> GGGAEALELLEHCGV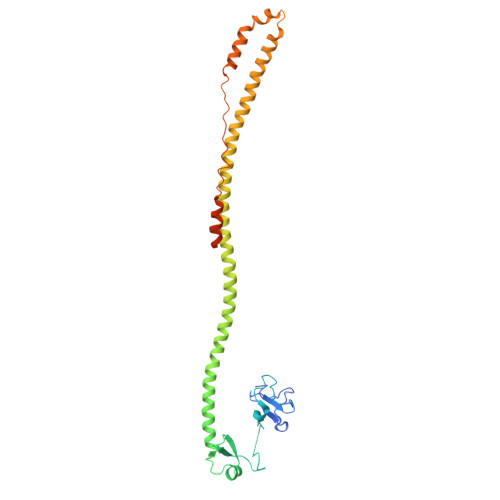CRERLRPEREPRLLPCLHSACSACLGPAAPAAANSSGDGGAAGDGTVVDCPVCKQQCFSKDIVENYFMRDSGSKAGERTVYCNVHKHEPLVLFCESCDTLTCRDCQLNAHKDHQYQFLEDAVRNQRKLLASLVKRLGDKHATLQKSTKEVRSSIRQVSDVQKRVQVDVKMAILQIMKELNKRGRVLVNDAQKVTEGQQERLERQHWTMTKIQKHQEHILRFASWALESDNNTALLLSKKLIYFQLHRALKMIVDPVEPHGEMKFQWDLNAWTKSAEAFGKIVAERPGTNSTGPAPMAPPRAPGPLSK> MKKLLVTVLLAVFGALAFAAEEAAASGGLDRGLIAVGMGLAVGLAALGTGVAQARIGAAGVGAIAEDRSNFGTALIFLLLPETLVIFG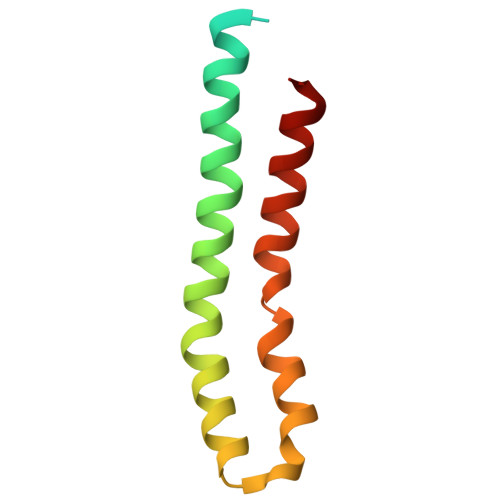LLIAFILNGRL>[2x]AHAFVSTLTRGDLSSIRWVCSSLRHAQPTCPG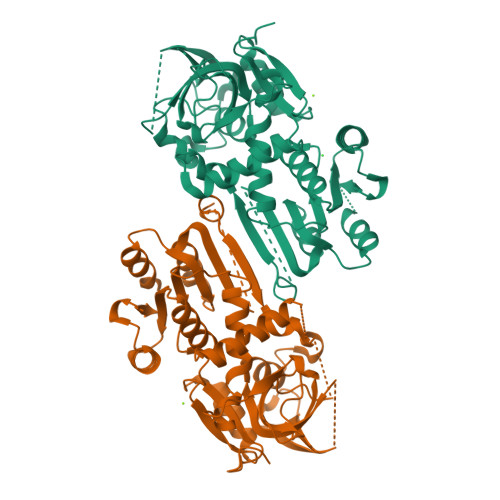AQLCTVYYASLNFRDIMLATGKLSPDAIPGKWTSQDSLLGMEFSGRDASGKRVMGLVPAKGLATSVLLSPDFLWDVPSNWTLEEAASVPVVYSTAYYALVVRGRVRPGETLLIHSGSGGVGQAAIAIALSLGCRVFTTVGSAEKRAYLQARFPQLDSTSFANSRDTSFEQHVLWHTGGKGVDLVLNSLAEEKLQASVRCLATHGRFLEIGKFDLSQNHPLGMAIFLKNVTFHGVLLDAFFNESSADWREVWALVQAGIRDGVVRPLKCTVFHGAQVEDAFRYMAQGKHIGKVVVQVLAEEPEAVLKG> RKKKRKDYQPNYFLSIPITNKEIIKGIKILQNAIIQQDERLAKAMVSDGSFHITLLVMQLLNEDEVNIGIDALLELKPFIEELLQGKHLTLPFQG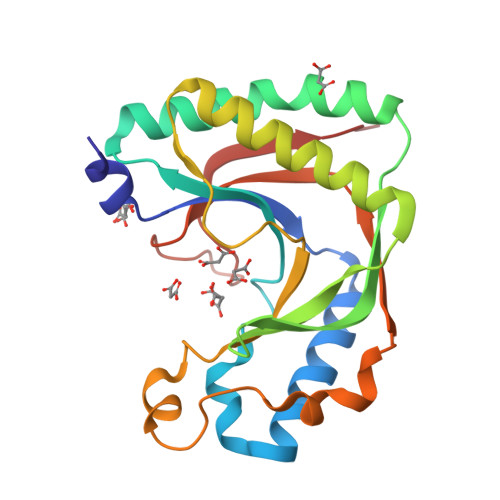IGTFGNQVGFVKLAEGDHVNSLLEIAETANRTFQEKGILVGESRSFKPHLTFMKLSKSPWLRKNGVKKIDPDLYEKFISHRFGEEILYRIDLCSMLKKKQSNGYYHCESSIVIGEK>MQLNNRDLKSIIDNEALAYAMYTVENRAIPNMIDGFKPVQRFVIARALDLARGNKDKFHKLASIAGGVADLGYHHGENSAQDAGALMANTWNNNFPLLDGQGNFGSRTVQKAAASRYIFARVSKNFYNVYKDTEYAPVHQDKEHIPPAFYLPIIPTVLLNGVSGIATGYATYILPHSVSSVKKAVLQALQGKKVTKPKVEFPEFRGEVVEIDGQYEIRGTYKFTSRTQMHITEIPYKYDRETYVSKILDPLENKGFITWDDACGEHGFGFKVKFRKEYSLSDNEEERHAKIMKDFGLIERRSQNITVINEKGKLQVYDNVVDLIKDFVEVRKTYVQKRIDNKIKETESAFRLAFAKAHFIKKVISGEIVVQGKTRKELTEE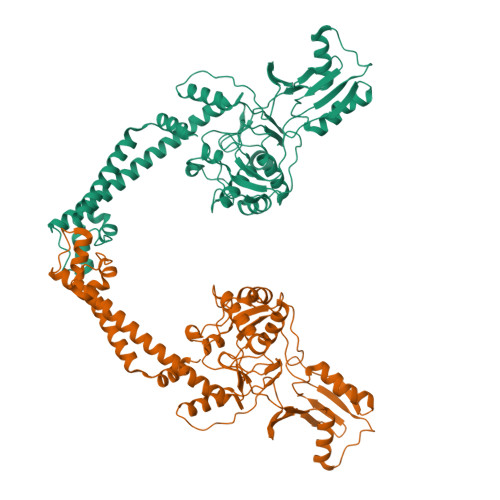LSKIDMYSSYVDKLVGMNIFHMTSDEAKKLAEEAKAKKEENEYWKTTDVVTEYTKDLEEIKHHHHHHHHHH[2x]N~3~-[(2R)-2-hydroxy-3,3-dimethyl-4-(phosphonooxy)butanoyl]-N-(5-methoxypentyl)-beta-alaninamide | C15 H31 N2 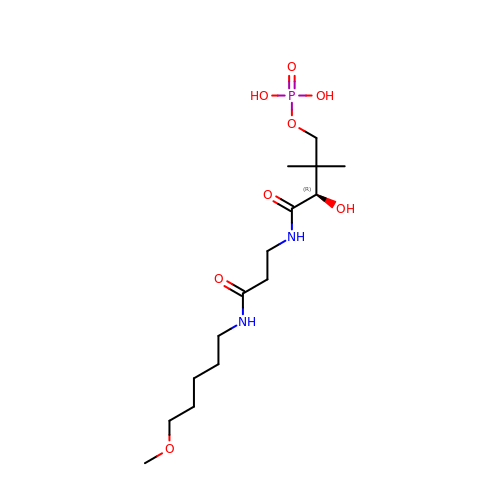O8 P | FOBYDOXAQNKICH-ZDUSSCGKSA-N PIE12-trimer is a highly potent d-peptide HIV-1 entry inhibitor that broadly targets group M isolates. It specifically binds the three identical conserved hydrophobic pockets at the base of the gp41 N-trimer with sub-femtomolar affinity. The target of PIE12 is the highly conserved pocket at the base of the gp41 N-trimer, a parallel trimeric coiled-coil region of gp41 that is transiently exposed (“prehairpin intermediate”) during HIV-1 entry. PIE12-trimer prevents the folding of the N-trimer and C-peptide regions of gp41 into the 6-helix bundle (trimer-of-hairpins) structure required for membrane fusion during viral entry, and it inhibits all members of a diverse panel of primary Group M HIV isolate strains with high pM to low nM potency (IC50).

Eventually, HIV developed resistance to PIE12-trimer by mutating Q577 in the gp41 pocket. Expanding on our earlier work that selected for viral resistance to PIE12-trimer, here we describe the biochemical, structural, and functional properties of the primary PIE12-trimer resistance mutations (Q577R/N/K). As in all previous d-peptide/IQN17 structures, IQN17 forms a continuous trimeric coiled coil with the d-peptide binding to the gp41 hydrophobic pocket region. In the WT structure, Q577 hydrogen bonds with d-Glu9 and d-Trp12 in PIE12. Q577R disrupts these hydrogen bonds, likely accounting for the loss of affinity, and induces a repositioning of two adjacent residues (d-Glu9 in PIE12 and L581 in IQN17, although d-Glu9 position is variable in the WT structures). Q577R disrupts two hydrogen bonds between PIE12-trimer and the inhibitor-binding pocket and substantially decreases binding affinity. The Q577R mutation results in a dramatic (~ 65-fold) weakening of the interaction between PIE12-monomer and the hydrophobic pocket (Q577R KD = 2.0 µM vs. 0.031 µM for WT), corresponding to a 2.5 kcal/mol weakening of the PIE12 interaction. Because our inhibitor is trimeric, we expect the impact on PIE12-trimer’s binding energy to be three times as great, corresponding to a geometric drop of binding affinity of 653 (or > 250,000). This large decrease in binding affinity is consistent with the prediction that an extremely disruptive mutation is required to overcome PIE12-trimer’s highly charged resistance capacitor. In an HXB2 pseudovirion, Q577R confers > 4000-fold resistance to PIE12-trimer. Q577 mutation confers a significant fitness defect as seen by delayed viral replication.

> XRMKQIEDKIEEIESKQKKIENEIARIKKLLQLTVWGIKQLRARILX;> XKGHPCDYPEWQWLCELX>MASGMIVTDAGADQPIVFVNRAFSTITGYAPNEVLGRNARFLQGPQTDAATVARLREAIAAARPIQERILNY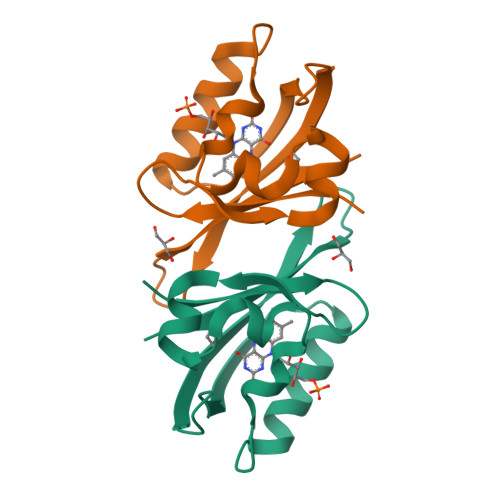RKDGQPFWNQLSISPVRDETGNVVAFVGVKTDVTAHHHHHH[2x]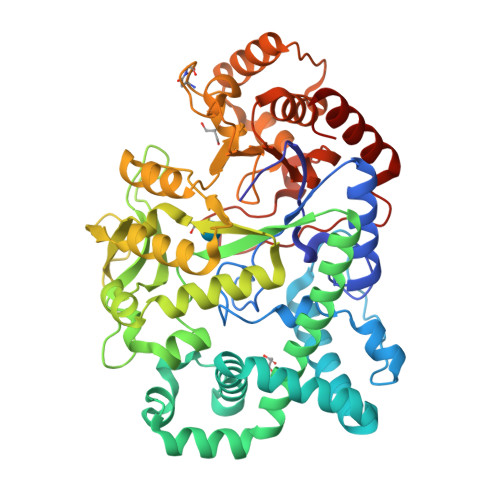> GSHMELPRAFGLLLHPTSLPGPYGVGVLGQEARDFLRFLKEAGGRYWQVLPLGPTGYGDSPYQSFSAFAGNPYLIDLRPLAERGYVRLEDPGFPQGRVDYGLLYAWKWPALKEAFRGFKEKASPEEREAFAAFREREAWWLEDYALFMALKGAHGGLPWNRWPLPLRKREEKALREAKSALAEEVAFHAFTQWLFFRQWGALKAEAEALGIRIIGDMPIFVAEDSAEVWAHPEWFHLDEEGRPTVVAGVPPDYFSETGQRWGNPLYRWDVLEREGFSFWIRRLEKALELFHLVRIDHFRGFEAYWEIPASCPTAVEGRWVKAPGEKLFQKIQEVFGEVPVLAEDLGVITPEVEALRDRFGLPGMKVLQFAFDDGMENPFLPHNYPAHGRVVVYTGTHDNDTTLGWYRTATPHEKAFMARYLADWGITFREEEEVPWALMHLGMKSVARLAVYPVQDVLALGSEARMNYPGRPSGNWAWRLLPGELSPEHGARLRAMAEATERL>GMSDLQSLQPKLLWQWFDQICAIPHPSYKEEQLAQFIINWAKTKGFFAERDEVGNVLIRKPATVGMENRKPVVLQAHLDMVPQANEGTNHNFDQDPILPYIDGDWVKAKGTTLGADNGIGMASALAVLESNDIAHPELEVLLTMTEERGMEGAIGLRPNWLRSEILINTDTEENGEIYIGCAGGENADLELPIEYQVNNFEHCYQVVLKGLRGGHSGVDIHTGRANAIKVLLRFLAELQQNQPHFDFTLANIRGGSIRNAIPRESVATLVFNGDITVLQSAVQKFADVIKAELALTEPNLIFTLEKVEKPQQVFSSQCTKNIIHCLNVLPNGVVRNSDVIENVVETSLSIGVLKTEDNFVRSTMLVRSLIESGKSY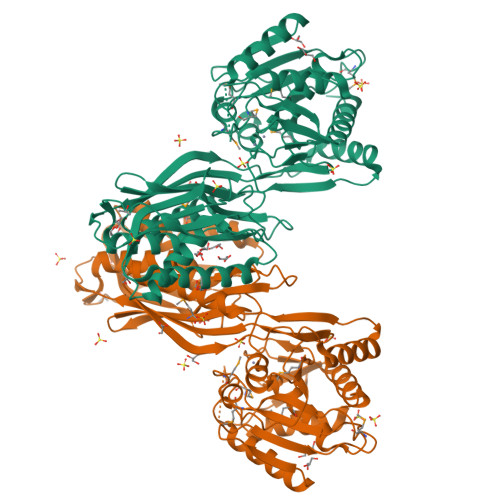VASLLKSLASLAQGNINLSGDYPGWEPQSHSDILDLTKTIYAQVLGTDPEIKVIHAGLECGLLKKIYPTIDMVSIGPTIRNAHSPDEKVHIPAVETYWKVLTGILAHIPSR[2x]> MFKKWKKFGISSLALVLVAAVAFTGWSAKASAADASQIVSEMGAGWNLGNQLEAAVNGTPNETAWGNPTVTPELIKKVKAAGFKSIRIPVSYLNNIGSAPNYTINAAWLNRIQQVVDYAYNEGLYVIINIHGDGYNSVQGGWLLVNGGNQTAIKEKYKKVWQQIATKFSNYNDRLIFESMNEVFDG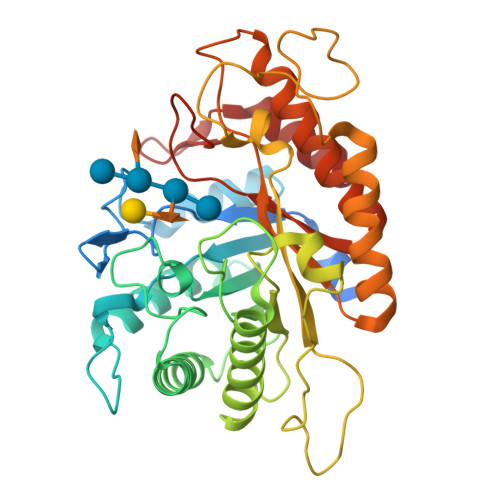NYGNPNSAYYTNLNAYNQIFVDTVRQTGGNNNARWLLVPGWNTNIDYTVGNYGFTLPTDNYRSSAIPSSQKRIMISAHYYSPWDFAGEENGNITQWGATSTNPAKKSTWGQEDYLESQFKSMYDKFVTQGYPVVIGEFGSIDKTSYDSSNNVYRAAYAKAVTAKAKKYKMVPVYWDNGHNGQHGFALFNRSNNTVTQQNIINAIMQGMQ>[10x]MHHHHHHGSDDDDKEQIDKQKIADAVKVILEAVGENPDREGLIDTPMRVARMYEEVFAGLKKDPSV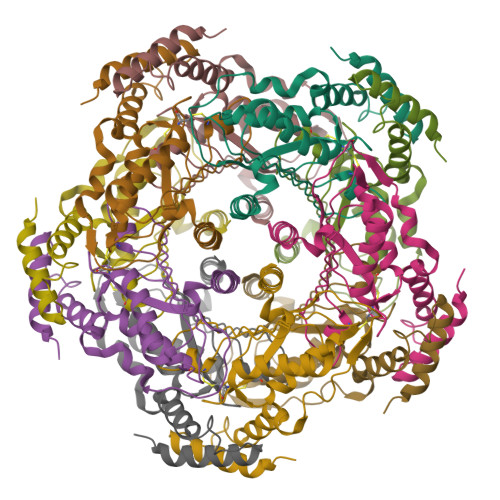HFDTIFEEQHEELVLVKDIRFSSMCEHHLVPFFGVAHVAYLPQNGRVAGLSKLARVVDDVSRRPQLQERITTTVAEIMMEKLKPLGVMVIMEAEHMCMTIRGVNKPGTKTITSAVRGAFKNDDKLRSEVLALIKHN>[2x]MSLANLSELPNIGKVLEQDLIKAGIKTPVELKDVGSKEAFLRIWENDSSVCMSEL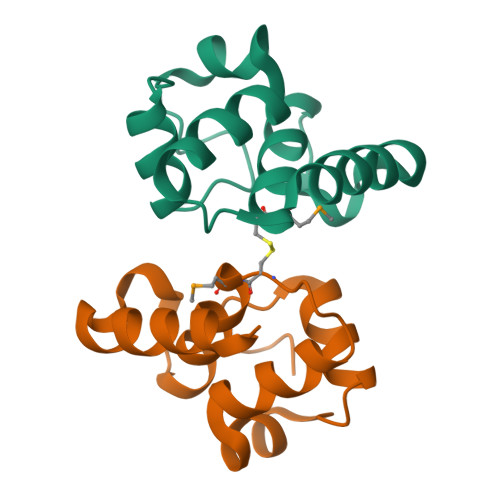YALEGAVQGIRWHGLDEAKKIELKKFHQSLEGHHHHHH>GMLESVRKEWLEIMDRELLE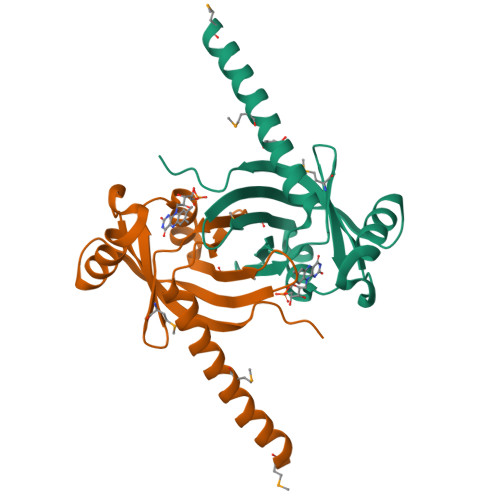KARSLINANYISTTLSTVDRNYEVNIAVISVLEMIGDDTIICARFGADKTYANLKETGKGVFMVLLTDNDKSKDGIRVYVELSADLQEGEYFDRIKKRLDNTTYKNFPLKNCLVFKIVKILPVSLLRK[2x]> APTAPSIDMYGSNNLQFSKIELAMETTSGYNDMVKYHELAKIKVKFNQWSGTSGDTYNVYFDGVKVATGAITGSQTTASFEYGQGGLYQMEIEACDATGCSKSAPVEITIADTDGSHLKPLTMNVDPNNKSYNTDPSIVMGTYFVEWGIYGRDYTVDNMPVDNLTHILYGFIPICGPNESVKSVGGNSFNALQTACRGVNDYEVVIHDPWAAYQKSFPQAGHEYSTPIKGNYAMLMALKQRNPDLKIIPSIGGWTLSDPFYDFVDKKNRDTFVASVKKFLKTWKFYDGVDIDWEFPGGGGAAADKGDPVNDGPAYIALMRELRVMLDELEAETGRTYELTSAIGVGYDKIEDVDYADAVQYMDYIFAMTYDFYGGWNNVPGHQTALYCGSFMRPGQCDGGGVDENGEPYKGPAYTADNGIQLLLAQGVPANKLVLGTAMYGRGWEGVTPDTLTDPNDPMTGTATGKLKGSTAQGVWEDGVIDYKGIKSFMLGANNTGINGFEYGYDAQAEAPWVWNRSTGELITFDDHRSVLAKGN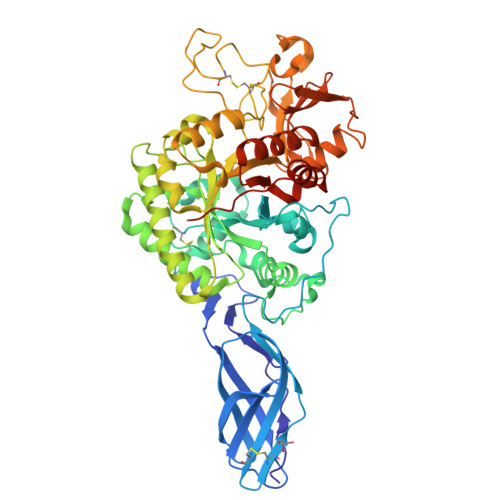YAKSLGLAGLFSWEIDADNGDILNAMHEGMAGGVVTPPNRRSHHHHHH>[2x]MISHIVAMDENRVIGKDNRLPWHLPADLAYFKRVTMGHAIVMGRKTFEAIGRPLPGRDNVVVTGNRSFRPEGCLVLHSLEEVKQWIASRADEVFIIGGAE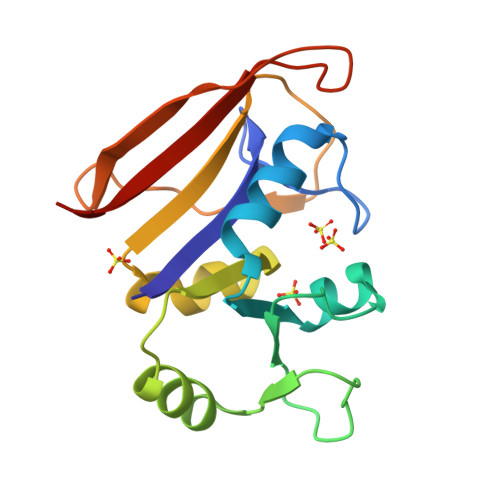LFRATMPIVDRLYVTKIFASFPGDTFYPPISDDEWEIVSYTPGGKDEKNPYEHAFIIYERKKAK>ALPTIHVVTPTYSRPVQKAELTRMANTLLHVPNLHWLVVEDAPRRTPLTARLLRDTGLNYTHLHVETPRNYKLRGDARDPRIPRGTMQRNLALRWLRETFPRNSSQ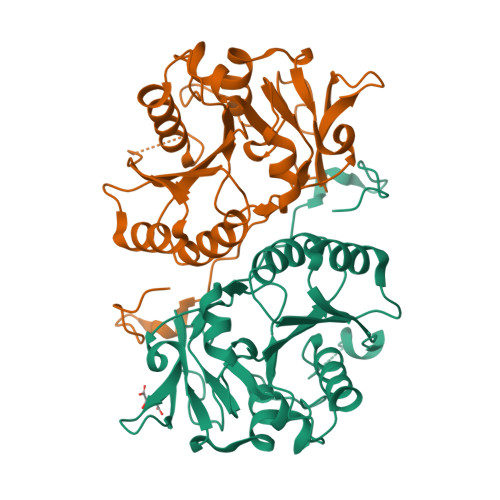PGVVYFADDDNTYSLELFEEMRSTRRVSVWPVAFVGGLRYEAPRVNGAGKVVRWKTVFDPHRPFAIDMAGFAVNLRLILQRSQAYFKLRGVKGGYQESSLLRELVTLNDLEPKAANCTKILVWHTRTEKPVLVNEGKKGFTDPSVEI[2x]(1~{S},3~{Z})-3-[(2~{E})-2-[(1~{R},3~{a}~{S},7~{a}~{R})-1-[(2~{R})-5,5-bis(fluoranyl)-6-methyl-6-oxidanyl-heptan-2-yl]-7~{a}-methyl-2,3,3~{a},5,6,7-hexahydro-1~{H}-inden-4-ylidene]ethylidene]-4-methylidene-cyclohexan-1-ol 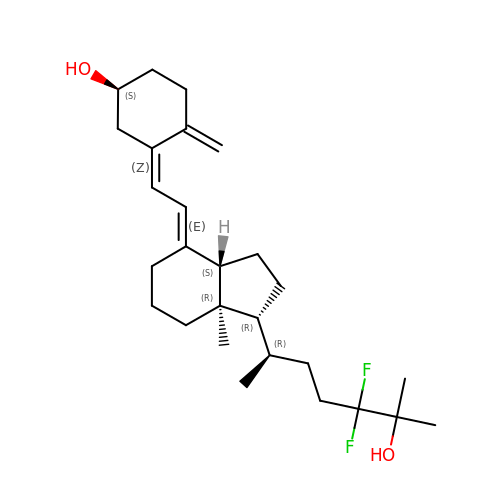| C27 H42 F2 O2 | LRNVEDCUBISUTC-CMOHYRQESA-N> AADVAGTSNRDFRGREQRLYNSEQYNYNNSLNGEVSLWVYAYYSDGSVLVRNCNSQYKVGISECFKSLKEVRVGQNNDPYDEQEVNNGVYYPNGGEPTKFHSNAKPRAIQIIFSPSVNVHTIKMAKGNSVSIPKDYLQRSHPWEATGVKYRKIHVDGEIVGYSHYFELPHEYNSISLSVSGVHKNPSSYNVAAPHNIMDVFQSCDLALKFSNRYWCELELINHYISAYAYPYLDINNHKYGVPLNGRQ

We use as an exemplar the successful structure determination of a novel polyhedrin from a cytoplasmic polyhedrosis virus (CPV) which infects the winter moth Operophtera brumata from our ongoing studies into polyhedra from insect viruses. Another engineered expression system, the baculovirus–Sf9 system, exploits the ability of the virus to induce the expression of the protein required for the production of viral inclusion bodies within insect cells. As expected, the structure of OpbrCPV18 polyhedrin is very similar (r.m.s.d. of 0.23 Å for all 248 Cα atoms) to that of BmCPV1, although there are several notable differences which will be reported elsewhere (Ji et al., in preparation). We have determined the structure of a novel cypovirus polyhedrin via in cellulo crystallography.

In this work, we present a novel approach whereby crystals are investigated in cellulo by mounting frozen live cells directly in the X-ray beam. The data obtained are of high quality, comparable to that obtained from isolated crystals, and enabled a facile structure determination. From a total of 40 in cellulo crystals identified from grid scans, 20 were integrated successfully by FastDP with the correct space group assigned. The 20 selected crystals displayed similar unit-cell parameters a = b = c = 103.04 Å, with a standard deviation of just 0.1 Å. BLEND determined that the inclusion of all crystals of a standard sufficient for automatic data integration produced an optimum data set in terms of both completeness and R value. Not only does the in cellulo approach reduce the time and effort required, it also maintains the samples in a biologically relevant environment, e.g. in the presence of other cellular components and under cellular ionic conditions. The workflow enabling the structure determination is both time-efficient and sample-efficient, and has produced high-quality data from significantly fewer crystals of only 4–5 µm in diameter, representing a crystal volume roughly an order of magnitude smaller than that of the crystals used for previous analyses. A clear benefit of the in cellulo method is the reduction in crystal handling, which minimizes manual effort and preserves the sample in a favourable and stable environment, as suggested by the unit-cell parameter observations.>[4x]MADPSHLLKHNASVDIDDSQGDDGSNHNDSFPLSSLANLFENEESSAPNEGVRSPQVPGDNKQNLRIRFQGPFRKGISNPMDLLESTIYESSAPKKAPMDSLFGYETYHHHPTENRRKRKKILLEKENLNSQAPSPDPPPVIKMFNRHMLFDIVSRGSTAELEGFLPFLLAQKKRLTDEEFREASTGKTCLTKALMNLNGGKNDTIPMLIDIAEKTGNLREFINSPFRDVYYRGQTALHIAIERRCKHYVELLVEKGADVHAQARGRFFQPKDEGGYFYFGELPLSLAACTNQPDIVHYLTENAHKKADIRRQDSRGNTVLHALVAIADNTRENTKFVTKVYDLLVIKCVKLYPDSSLEAIFNNDSMSPLMMAAKLGKIGIFQHIIRLEIKDEEARHLSRKFRDWAYGPVYSSLYDLSMLDTCGEEVSVLEILVYNSKVENRHEMLAVEPINELLRDKWQKFGAVSFYISVVSYLIAMIIFTLIAYYRPM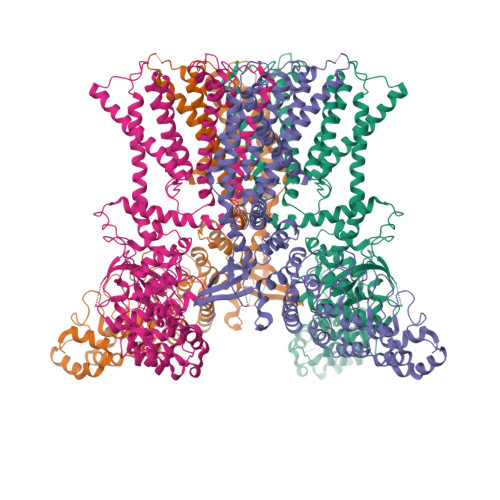DGTPPYPYRTTMDYMRLAGEIVTLLTGVVFFITNIKDLFMKKCPGVNSLFIDGSFQLLYFIYSVLVIITAVLYLVGIESYLAVMVFALVLGWMNALYFTRGLKLTGTYSIMLQKILFKDLFRFLLVYLLFMIGYASALVSLLNPCTSQESCIETSSNCTVPEYPSCRDSSTFSKFLLDLFKLTIGMGDLEMINSAKYPAVFIILLVTYIILTFVLLLNMLIALMGETVGQVSKESKQIWKLQWATTILDIERSFPVCMRKAFRSGEMVTVGKNLDGTPDRRWCFRVDEVNWSHWNQNLGIINEDPGRNDGYQYYGFSQTVGRLRRDRWSVVVPRVVELNKAPQHSDDVVVPLGNIPQVQTYSQRQENAQNWKKDETHI>[2x]SMFSGVVDIIVVRQPDDSLKSMPFHIRFGTLKVLDNQNINIQITVNDKKIEDVFMLMLPEGACYFPELNAKNEIQKKLRPSSAILKKFNLKNGYNKIQFIAESDLQGKQLIEGKIYLYNYDTKLVISDVDGTVTKSDVKGHISTIIGKEWTHDDIAELYTNIQK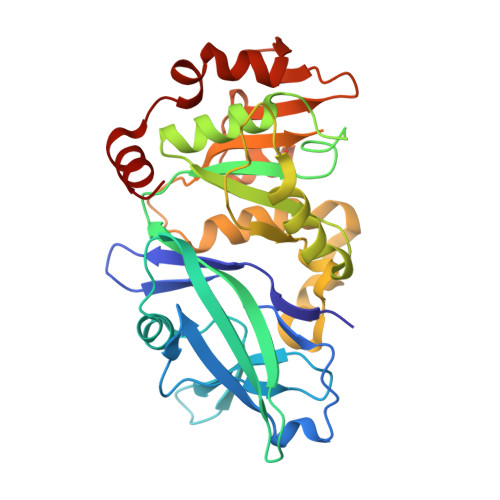NGYKMVYLSSRPLYFYNYTQGYLKGIIQNGFTMPDGPILLSPDQIISSLNREVVYKKADEFKGALLKDLRRVFPEEVNPIFAGFGNRDTDATACLYAGVIIDNIFIINEQSQVEILGKQEKSSYKKINEKIQELFPRLPAAALEHHHHH> MYATKPGLARLAPAVLAAAVFVATPGTADAHAHLRAADPPEAIVDAAGLREIRLVFSEPVVDRFSTFRAFRLSLPENGIRNLTQLNTLASELGVDTEESAHHEVELESDLSSQSAE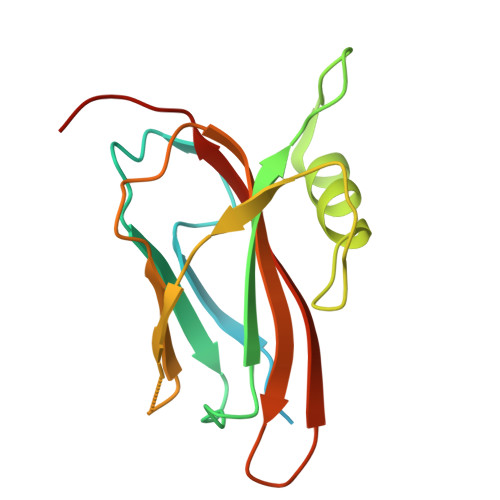VTLHSDEPLPAGAYAVVWRVLSVDGHTTTGFHAFVHAGGTASSH> GSARGCHIAQFKSLSPRELQAFKRAKDALEESLLLKDCKCRSRLFPRTWDLRQLQVRERPVALEAELALTLKVLDATADTDPALGDVLDQPLHTLH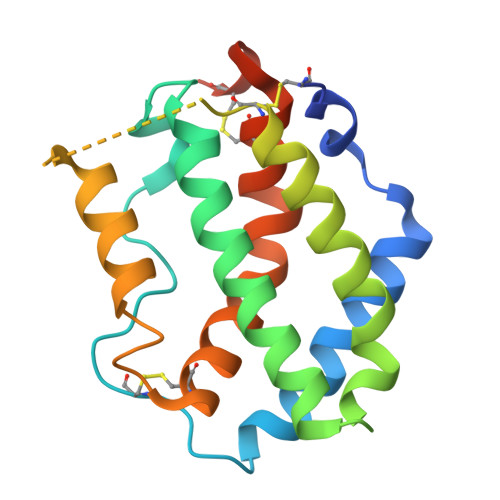HILSQLRACIQPQPTAGPRTRGRLHRWLHRLQEAPKKESPGCLEASVTFNLFRLLARDLNCVASGDLCEAAAHHHHHHHH Lipoprotein(a) (Lp(a)), an independent, causal cardiovascular risk factor, is a lipoprotein particle that is formed by the interaction of a low-density lipoprotein (LDL) particle and apolipoprotein(a) (apo(a)). Lp(a) is a lipoprotein particle that is formed by a two-step process involving interactions between a LDL particle and another protein, apo(a). The goal of our research was to develop a potent and selective orally delivered small-molecule therapeutic to inhibit the formation of Lp(a) by blocking the first interaction between apo(a) and apoB to reduce the circulating levels of Lp(a). In summary, we report the discovery and optimization of potent and selective small-molecule inhibitors of Lp(a) formation by exploiting the repeated KIV domain structure of apo(a) through compound multivalency.

The linkage of two molecules that contain the crucial LSN3353871 KIV domain interaction motif created a dimeric molecule, LSN3441732. This dimeric compound inhibits the formation of Lp(a) particles in vitro with an IC50 value of 0.18 nM (n = 8), representing an increase in potency of three orders of magnitude compared with the parent monomeric molecule, LSN3353871 (IC50 = 1.69 µM; n = 43) and two orders of magnitude compared with an optimized monomeric ligand, LSN3374443 (IC50 = 36 nM; n = 3). In direct binding assays, 3H-LSN3374443 bound to full-length recombinant apo(a) with a mean Kd value of 2.6 nM and an approximate maximum saturable binding (Bmax) value of 9.8 fmol ng−1 apo(a), equivalent to two to three ligands per molecule of apo(a). In comparison, 3H-LSN3441732 bound to full-length apo(a) with a 50-fold affinity increase of Kd = 0.05 nM and with Bmax = 4.9 fmol ng−1 apo(a), indicative of one ligand per molecule of apo(a). Notably, as observed with the monomeric compound LSN3353871, binding of LSN3441732 to KIV2 was ruled out using ITC. In Lp(a) transgenic mice, LSN3441732 plasma concentrations increased in a dose-dependent manner and steady-state plasma Lp(a) levels decreased after five days of oral BID dosing, with an ED50 of 4 mg kg−1 and a mean maximal inhibition of 79% at the 30 mg kg−1 dose. In cynomolgus monkeys, 2 mg kg−1 and 10 mg kg−1 oral BID doses of LSN3441732 decreased median Lp(a) levels by a maximum of 45% and 57%, respectively, after 5 days of dosing, and continued to suppress the steady-state levels of Lp(a) for 14 days. Compatible with a multivalent binding mechanism, LSN3441732 showed improvements in potency and efficacy both in vitro and in vivo compared with the monovalent inhibitor.

>[2x]MAPTEQSPTVQDCYHGDGQSYRGSFSTTVTGRTCQSWSSMTPHWHQRTTEYYPNGGLTRNYCRNPDAEIRPWCYTMDPSVRWEYCNLTQCPVMEST>KRCSCSSLMDK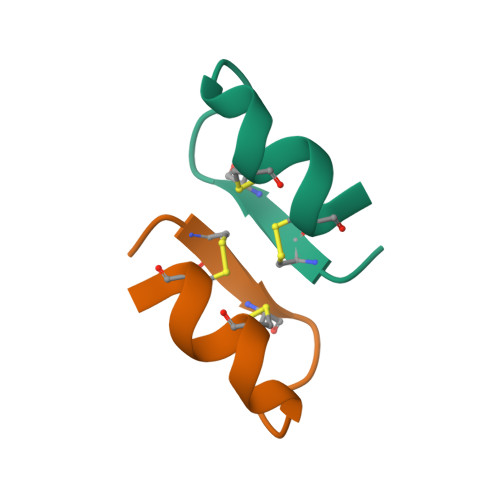ECVYFCH[2x]>[2x]MLQPFAWQVASLADRYEESFDIGAAVEPHQLNGRQGKVLKHHYNSIVAENAMKPISLQPEEGVFTWDGADAIVEFARKNNMNLRFHTLVWHNQVPDWFFLDEEGNPMVE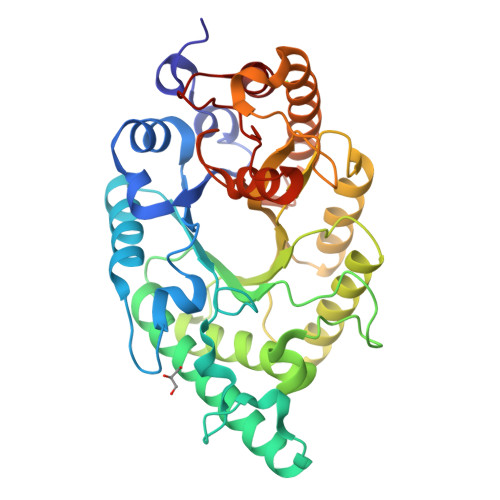ETNEAKRQANKELLLERLETHIKTVVERYKDDVTAWDVVNEVVDDGTPNERGLRESVWYQITGDEYIRVAFETARKYAGEDAKLFINDYNTEVTPKRDHLYNLVQDLLADGVPIDGVGHQAHIQIDWPTIDEIRTSMEMFAGLGLDNQVTELDVSLYGWPPRPAFPTYDAIPQERFQAQADRYNQLFELYEELDADLSSVTFWGIADNHTWLDDRAREYNDGVGKDAPFVFDPNYRVKPAFWRIID> MNSRPAEKIDNNDGQTETPRSKTVSTINSTDALAMVEHSSELTLSITTPVGTKFVCRTPFIGTHTDKFLLVEMPKISADDLQYFFQEGFWMNIRAISPRGEGALIHFRSQLMHILQEPVPMAFLSIPNTMQVSQLRKEPRFELNLAGKVLFDEHRGDCELRDLSRSGCRFITPPLGKTYQVGDLVALEIFSDLRGTKTFPPLTGKICNLQRSLHHARYGLEFNEEGRNNAKNLLAQLKFNGTKLTLN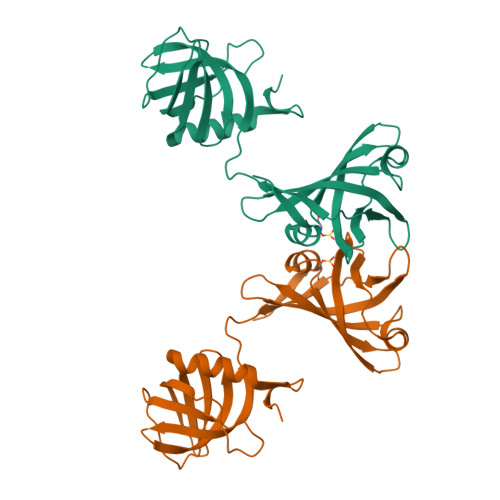AEKKA>MAGSHHHHHHTDPTGATFPEEAIADLSVNMYNRLRATGEDENILFSPLSIALAMGMMELGAQGSTQKEIRHSMGYDSLKNGEEFSFLKEFSNMVTAKESQYVMKIANSLFVQNGFHVNEEFLQMMKKYFNAAVNHVDFSQNVAVANYINKWVENNTNNLVKDLVSPRDFDAATYLALINAVYFKGNWKSQFRPENTRTFSFTKDDESEVQIPMMYQQGEFYYGEFSDGSNEAGGIYQVLEIPYEGDEISMMLVLSRQEVPLATLEPLVKAQLVEEWANSVKKQKVEVYLPRFTVEQ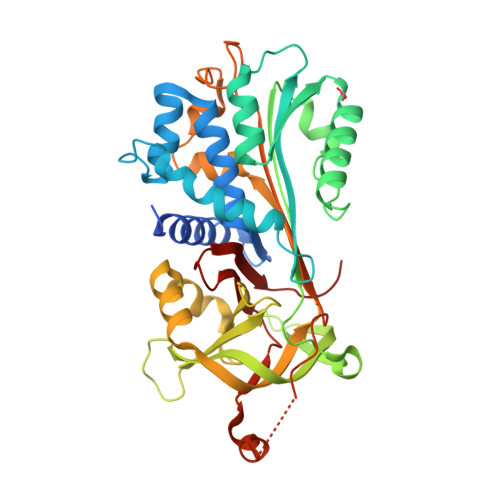EIDLKDVLKALGITEIFIKDANLTGLSDNKEIFLSKAIHKSFLEVNEEGSEAAAVSGMIAISRMAVLYPQVIVDHPFFFLIRNRRTGTILFMGRVMHPETM[2x]> MH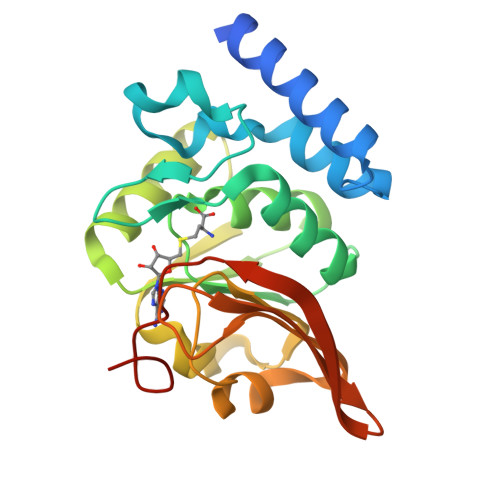LYSSDFPLMMDEKELYEKWMRTVEMLKAEGIIRSKEVERAFLKYPRYLSVEDKYKKYAHIDEPLPIPAGQTVSAPHMVAIMLEIANLKPGMNILEVGTGSGWNAALISEIVKTDVYTIERIPELVEFAKRNLERAGVKNVHVILGDGSKGFPPKAPYDVIIVTAGAPKIPEPLIEQLKIGGKLIIPVGSYHLWQELLEVRKTKDGIKIKNHGGVAFVPLIGEYGWKEHHHHHH>GPGSMIQTVVKRDGRIVGFNEQKIMAAIRKAMLHTDKGEDTTLIEQITDHISYRGKSQMSVEAIQDAIEMELMKSARKDVAQKYIAYRNQRNIARKAKTRDVFMSIVNAKNNDITRENANMNADTPAGMMMKFASETTKPFVDDYLLSEDVRDAVMHNYIHIHDKDYYPTKSLTCVQHPLDVILNHGFTAGHGSSRPAKRIETAAVLACISLETCQNEMHGGQAIPAFDFYLAPYVRMSYQEEVKNLEKLTGEDLSNLYDAPIDDYIEKPLDGLQGRERLEQHAINKTVNRVHQAMEAFIHNMNTIHSRGGNQVVFSSINYGTDTSAEGRCIMREILQSTYQGVGNGETAIFPIQIWKKKRGVNYLPEDRNYDLYKLACKVTARRFFPNFLNLDATFNQNEKWRADDPERYKWEIATMGCRTRVFEDRWGEKTSIARGNLSFSTINIVKLAIECMGIENEKQRIDMFFAKLDNILDITAKQLDERFQFQKTAMAKQFPLLMKYLWVGAENLKPEETIESVINHGTLGIGFIGLAECLVALIGKHHGESEKAQELGLKIITYMRDRANEFSEQYHHNYSILATPAEGLSGKFTKKDRKQFGVIPGVTDRDYYTNSNHVPVYYKCTALKKAQIEAPYHDLTRGGHIFYVEIDGDATHNPSVIESVVDMMDKYNMGYGSVNHNRNRCLDCGYENADAHLEVCPKCGSHHIDKLQRITGYLVGTTDRWNSGKLAELHDRVTHIGGEK[2x]

RNRs produce all four deoxyribonucleotides and are the only enzymes providing de novo building blocks for DNA replication and repair in all free-living organisms. Class III RNRs, which only function anaerobically, are dimers of an α subunit (NrdD) with a stable radical close to the active site, and binding sites for allosteric nucleotides. Binding of ATP activates RNR, and binding of dATP inhibits it. Here, we present structural, biochemical, and biophysical studies on the ATP-cone-containing NrdD from the human pathogen Prevotella copri (PcNrdD; Nii et al., 2023), showing that the binding of dATP causes increased flexibility of the C-terminal glycyl radical-bearing domain, as well as a flap-like loop that binds across the top of the active site in the active form.

Two-dimensional (2D) classes of particles extracted from micrographs of PcNrdD incubated with effector ATP and substrate CTP indicated only dimers, with no appreciable amounts of tetramer. As the ATP-cone density still did not permit reliable modelling, three-dimensional (3D) classification was carried out on this particle set, enabling the identification of a subset of 291,231 particles that gave a volume at 3.2 Å with better-defined ATP-cones. The ATP-cones containing the a-site are flexible, but the reconstruction from a subset of particles allowed the modelling of two ATP molecules per ATP-cone and many of the most important side chains. However, the ATP-cones in PcNrdD exhibit a hitherto unobserved relative orientation in which the four triphosphate groups are projected towards each other. Strikingly, the dimer of ATP-cones is slightly offset from the dimer axis of the core protein, such that the ATP-cone of the inactive monomer approaches the core domain of the active monomer, while the ATP-cone of the active monomer is more distant from the core domain of the inactive one. Two residues from the flap make H-bonds to CTP: Asn114 to the γ-phosphate group and Asn116 to the amino group of the cytosine base. Significantly, the NxN flap forms the nexus of a network of interactions between the substrate, the linker to the ATP-cone, the C-terminal GRD, and ‘loop 2’ (residues 304–311) that is responsible for communicating the substrate specificity signal from the s-site at the dimer interface to the active site. Important interactions linking the NxN flap to the C-terminus include H-bonds from Tyr712, which immediately follows the radical Gly711, to Glu581, which bridges to both the substrate and Ala115 in the flap, as well as from Arg719 in the GRD to the main chain carbonyl groups of Asn114 and Met117 in the flap. As the NxN flap appears to close off the top of the active site, we used the web server Caver Web v1.1 to analyse substrate access to the active site in the ATP-bound form, and identified a tunnel ~12 Å long leading from the surface of the protein to the active site that is 5.6 Å in diameter at its narrowest point.> MRGSHHHHHHGSMSQPDATPFDYILSGGTVIDGTNAPGRLADVGVRGDRIAAVGDLSASSARRRIDVAGKVVSPGFIDSHTHDDNYLLKHRDMTPKISQGVTTVVTGNCGISLAPLAHANPPAPLDLLDEGGSFRFARFSDYLEALRAAPPAVNAACMVGHSTLRAAVMPDLRREATADEIQAMQALADDALASGAIGISTGAFYPPAAHASTEEIIEVCRPLITHGGVYATAMRDEGEHIVQALEETFRIGRELDVPVVISHHKVMGKLNFGRSKETLALIEAAMASQDVSLDAYPYVAGSTMLKQDRVLLAGRTLITWCKPYPELSGRDLEEIAAERGKSKYDVVPELQ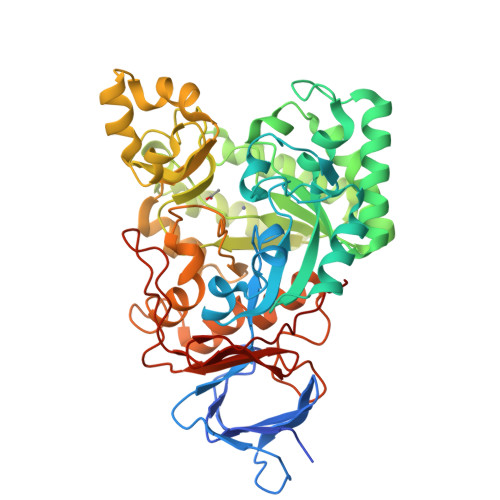PAGAIYFMMDEPDVQRILAFGPTMIGSDGLPHDERPHPRLWGTFPRVLGHYSRDLGLFPLETAVWKMTGLTAAKFGLAERGQVQPGYYADLVVFDPATVADSATFEHPTERAAGIHSVYVNGAAVWEDQSFTGQHAGRVLNRAGA Here we report the synchronous behavior of the adenine riboswitch aptamer RNA in crystal during ligand-triggered isothermal phase transitions. Here we report the interplay of synchronous molecular conformational changes and ordered SS transitions in crystals of adenine riboswitch aptamer RNA (riboA), elucidated using a multidisciplinary approach. Using a combination of methods—PVM, AFM, and XFEL—the results of this study demonstrate, in real time, the synchrony of molecular changes that occur in the ligand-induced phase transition of riboA crystals.

The first transition, AUC to TUC1, is measurable by the change in the c-axis from 9.3 to 7.9 nm. The phase transition from TUC1 to BUC, however, is slow enough to observe an intermediate topography (Fig. 2a (image #119), b (image #119 and #120) and Supplementary Table 1). One portion of image #119 corresponds to TUC1 topo 2, which is similar to the preceding AFM image; another portion (white box) corresponds to BUC topo 1, which is similar to the succeeding AFM image. A third portion (green box), which is sandwiched in between, exhibits a topography that is distinct from either, and whose autocorrelation plot gives a c-axis measurement of ~12.5 nm. Mixed lattices in transition (AUC and TUC1), as well as a unique lattice (TUC2) with a c-axis of 12.4 nm, were observed in X-ray diffraction experiments (see the next section). In particular, the c-axis measurement (~12.5 nm) observed in the TUC1–BUC intermediate (image #119) was used to guide the indexing of diffraction data. TUC2, with a c-axis of 12.4 nm, was identified in a small population (500 crystals) of the mixing data (up to 175 s), and in a greater population (3770 crystals) in a separate pool of data collected from sample premixed with ligand (>7 min post mixing). Based on the sequential appearance in both PVM and AFM, T1 observed by PVM corresponds to the AUC–TUC1 lattice transition, whereas T2 and T3 are likely related to the transitions from TUC1 to TUC2, and from (TUC1/TUC2) to BUC.

>GGGAAGAUAUAAUCCUAAUGAUAUGGUUUGGGAGUUUCUACCAAGAGCCUUAAACUCUUGAUUAUCUUCCC[2x]> SGHVKRPMNAFMVWARIHRP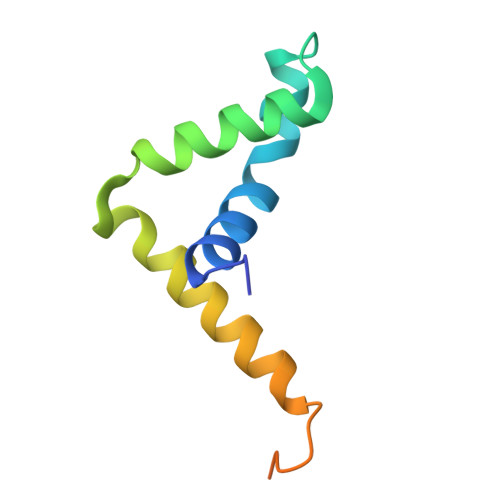ALAKANPAANNAEISVQLGLEWNKLSEEQKKPYYDEAQKIKEKHREEFPGWVYQPRPGKRKRFPLSVSNV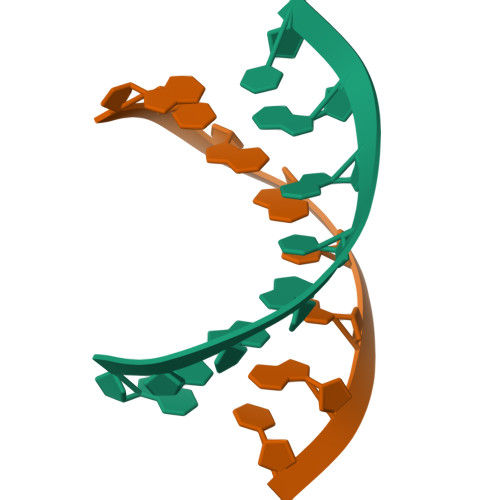>[36x]GCGGCGGC>[5x]GSHMGGVEVLEVKTGVDSITEVECFLTPEMGDPDEHLRGFSKSISISDTFESDSPNRDMLPCYSVARIPLPNLNEDLTCGNILMWEAVTLKTEVIGVTSLMNVHSNGQATHDNGAGKPVQGTSFHFFSVGGEALELQGVLFNYRTKYPDGTIFPKNATVQSQVMNTEHKAYLDKNKAYPVECWVPDPTRNENTRYFGTLTGGENVPPVLH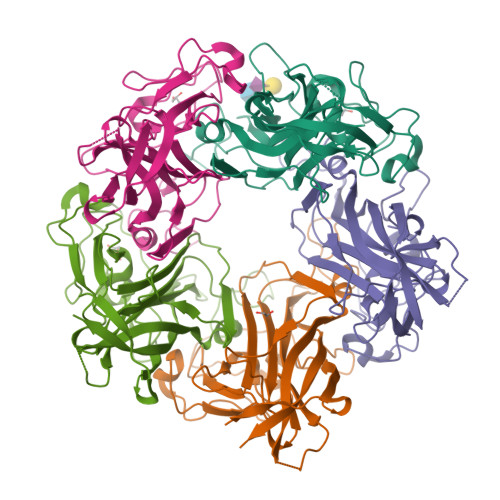ITNTATTVLLDEFGVGPLCKGDNLYLSAVDVCGMFTNRSGFQQWRGLSRYFKVQLRKRRVKN> GPGTNRSLIVTTLLEEPFVMFRKSDRTLYGNDRFEGYCIDLLKELAHILGFSYEIRLVEDGKYGAQDDKGQWNGMVKELIDHKADLAVAPLTITHVREKAIDFSKPFMTLGVSILYRKGTPIDSADDLAKQTKIEYGAVKDGATMTFFKKSKISTFEKMWAFMSSKPSALVKNNEEGIQ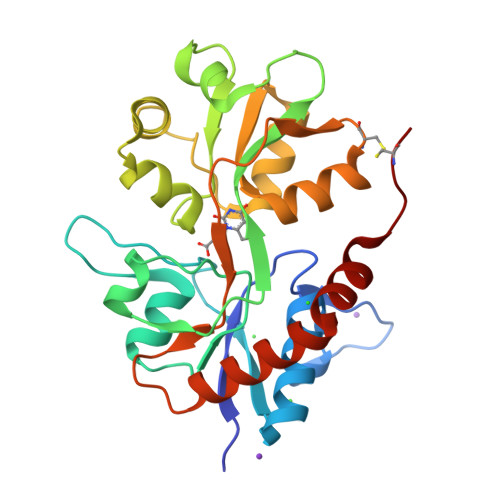RTLTADYALLMESTTIEYITQRNCNLTQIGGLIDSKGYGIGTPMGSPYRDKITIAILQLQEEDKLHIMKEKWWRGSGCP URIDYLYL-2'-5'-PHOSPHO-GUANOSINE | C19 H24 N7 O13 P | 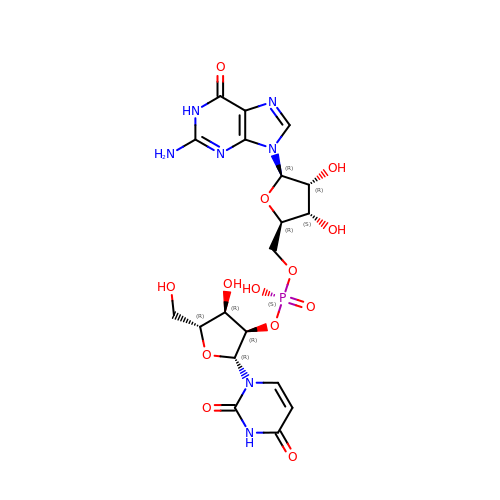DFYLLEBFVZTKHD-VMIOUTBZSA-N> MSQVAALLIALPLISAFFVPVLKQIGKSLIKPFLVIITLLQTLIASWAFVQVYSTGKPIIIYAGGWKPPIGINLYIGHFAALFILVIAVVSFLMALFNFKAVTVEPIDKYAMLFLLLLLGATGMIATGDIFNLFVFMEITAISAYALTAYNKTGEAAEASMKYIVLGGIGSSFFLVGVALIYGATGTLNMAHLAMLANDINPTVVQVGLALIIFGLAVEAELFPLNAWAPDAYQAAPHPITVMFSAFVVKAGLYAMARILYLFKDVSGWSSLTKLLIAMATLTVVFAELSALRQKNVKRMIAYSSIGQ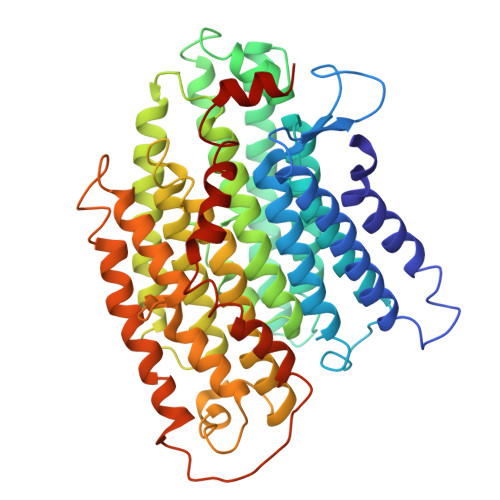VGLIALALSLGTQEGVSAGVFHMLNHAIVKTMMFMAIGYVGITLGGTMIENFEGLGKRMPLTSLSLTIGGIATVGVPLFNVFWSKLRIILAAAHEGNLWPVALVLFASVVEAVYYFRLIHTMWFKGKSGERIPEGAIAIVLLLLAMLIIVIGVYPTPFWNLVTKAGSDIVEVSKYVANVLPGVKL>[4x]GPGSMTDFYSLIPSAPKGRFDGIERAHTAEDVKRLRGSVEIKYSLAEMGANRLWKLIHEEDFVNALGALSGNQAMQMVRAGLKAIYLSGWQVAADANTASAMYPDQSLYPANAGPELAKRINRTLQRADQIETAEGKGLSVDTWFAPIVAD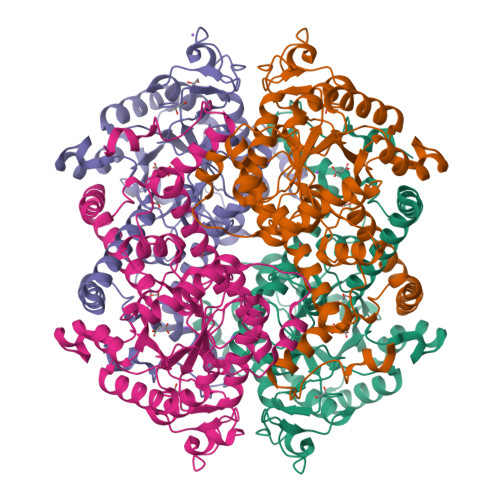AEAGFGGPLDAFEIMKAYIEAGAAGVHFEDQLASEKKCGHLGGKVLIPTAAHIRNLNAARLAADVMGTPTLIVARTDAEAAKLLTSDIDERDQPFVDYEAGRTAEGFYQVKNGIEPCIARAIAYAPYCDLIWMETSKPDLAQARRFAEAVHKAHPGKLLAYNCSPSFNWKKNLDDATIAKFQRELGAMGYKFQFITLAGFHQLNYGMFELARGYKDRQMAAYSELQQAEFAAEADGYTATKHQREVGTGYFDAVSLAITGGQSSTTAMKESTETAQFKPAAE>[2x]MSVTVPNDDWTLSSLSETF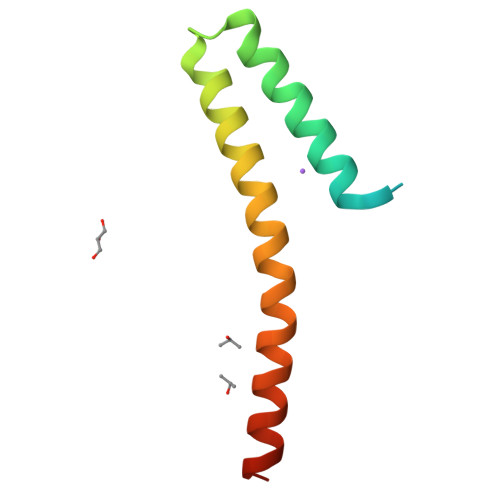DDGTQTLQGELTLALDKLAKNPSNPQLLAEYQSKLSEYTLYRNAQSNTVKVIKDVDAAILEHHHHH> KDHQLL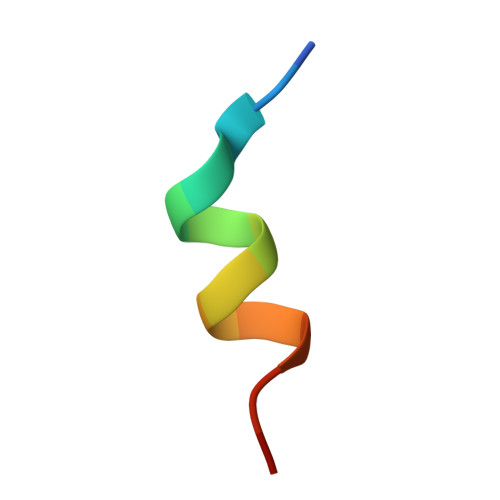RYLLDKDE The heterotrimeric [FeFe] hydrogenase, HydABC, from T. maritima is a soluble cytoplasmic enzyme involved in fermentation. It uses electrons from the one-electron carrier ferredoxin (E°′ ≈ −450 mV Schut and Adams, 2009), which is reduced during pyruvate metabolism, and the two-electron carrier NADH (E°′ ≈ −20 mV; Schut and Adams, 2009), produced during glucose metabolism, to reduce protons to hydrogen (E°′ ≈ −420 mV; Schut and Adams, 2009). The electron-bifurcating [FeFe] hydrogenase from Thermotoga maritima (HydABC) requires both NADH and ferredoxin to reduce protons generating hydrogen. Electron bifurcation is a fundamental energy conservation mechanism in nature in which two electrons from an intermediate-potential electron donor are split so that one is sent along a high-potential pathway to a high-potential acceptor and the other is sent along a low-potential pathway to a low-potential acceptor.

To further explore the particles without a bridge a further classification was used. It was possible to obtain a low-resolution map of a class where the HydB CT domain was found in an ‘open’ conformation. Fourier shell correlation (FSC) curves showing the resolution of (A, B) the ‘bridge closed’ maps, both reaching a resolution of 2.8 Å and (C), the ‘bridge open’ map, reaching a resolution of 2.7 Å (although note that the bridge is much less well resolved than the core in this particular map). We identified two conformations of a flexible iron–sulfur cluster domain: a ‘closed bridge’ and an ‘open bridge’ conformation, where a Zn2+ site may act as a ‘hinge’ allowing domain movement. Using symmetry expansion, we have also observed two conformations of the HydB-CT domain, a domain that is unique to and conserved in bifurcating hydrogenases, consistent with mechanistically relevant conformational changes.

> MKIYVDGREVIINDNERNLLEALKNVGIEIPNLCYLSEASIYGACRMCLVEINGQITTSCTLKPYEGMKVKTNTPEIYEMRRNILELILATHNRDCTTCDRNGSCKLQKYAEDFGIRKIRFEALKKEHVRDESAPVVRDTSKCILCGDCVRVCEEIQGVGVIEFAKRGFESVVTTAFDTPLIETECVLCGQCVAYCPTGALSIRNDIDKLIEALESDKIVIGMIAPAVRAAIQEEFGIDEDVAMAEKLVSFLKTIGFDKVFDVSFGADLVAYEEAHEFYERLKKGERLPQFTSCCPAWVKHAEHTYPQYLQNLSSVKSPQQALGTVIKKIYARKLGVPEEKIFLVSFMPCTAKKFEAEREEHEGIVDIVLTTRELAQLIKMSRIDINRVEPQPFDRPYGVSSQAGLGFGKAGGVFSCVLSVLNEEIGIEKVDVKSPEDGIRVAEVTLKDGTSFKGAVIYGLGKVKKFLEERKDVEIIEVMACNYGCVGGGGQPYPNDSRIREHRAKVLRDTMGIKSLLTPVENLFLMKLYEEDLKDEHTRHEILHTTYRPRRRYPEKDVEILPVPNGEKRTVKVCLGTSCYTKGSYEILKKLVDYVKENDMEGKIEVLGTFCVENCGASPNVIVDDKIIGGATFEKVLEELSKNG;> MFKNAKEFVQYANKLKTLREKKLNGVSIYVCVGTGCTAKGALKVYSAFEEELKKRNLLGQVTLEKIDDDKVTLNRTGCCGRCSSGPLVKIMPYRFFYSNVAPEDVPEIVDRTVLKGEPIERLFLTDPLTGEKVPRIEDTTLFKNQDFYIMEAIGESECDSIEDYIARSGYESLVKALTSMTPEEIIETVKASGLRGRGGGGFPTGLKWEFTRKAQGDIKFVVCNGDEGDPGAFMNRTLLERDPHLVLEGMIIAGYAVGAQKGYAYIRAEYPFAVKMFKKAIEDARKLGLLGENILGTGFSFDLEVKEGAGAFVCGEETALLASIEGKRGMPRPKPPFPAQSGLWGKPTLINNVETYANIPRILRDGVENYRKRGTENSPGTKMFSVAGPLKATGIIEVEFGTTLRDIIYNICGGFVEGEEFKAVQIGGPSGACLSEDFIDMPLDYDTLKKADAMVGSGGIVVITKKTCMVEVARFFLDFTKRESCGKCVPCREGTMQAYNILEKFTHGKATYEDLKTLEHLSKTIKTASLCGLGKTAPNPILSTLKLFREEYIAHIEGECPSGMCTAFKKYVINPDICKGCGLCARSCPQNAITGERGKPYTIDQEKCVKCGLCASKCPFKAIELV;> MASWSHPQFEKSGGGGGENLYFQGAVLALERHFEKVEEILKKYGYKRENLIKILLEIQEIYRYLPEDVINYVSTAMGIPPAKIYGVATFYAQFSLKPKGKYTIMVCDGTACHMAGSPEVLKAIEEETGLTPGNVTEDLMFSLDQVGCLGACALAPVMVINGEVYGNLTADKVKEILRKIKEKERESANV> ATQSPGDSRRLSIQRAIQSLVHAAQCRNANCSLPSCQKMKRVVQHTKGCKRKTNGGCPICKQLI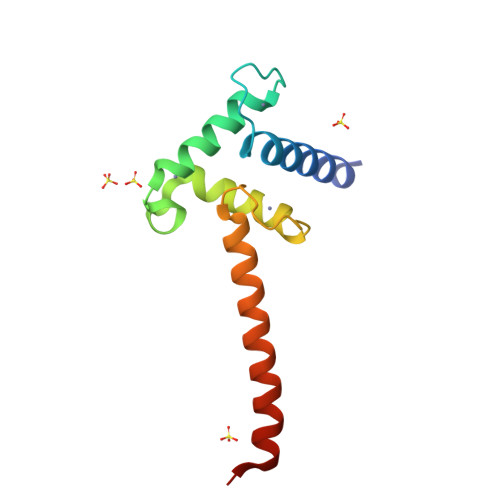ALAAYHAKHCQENKCPVPFCLNIKQKLRQQQLQHRLQQAQMLRRRMASMQ>SLINTKIKPFKNQAFKNGEFIEVTEKDTEGRWSVFFFYPADFSFVCPTELGDVADHYEELQKLGVDVYSVSTDTHFTHKAWHSSSETIAKIKYAMIGDPTGALTRNFDNMREDEGLADRATFVVDPQGIIQ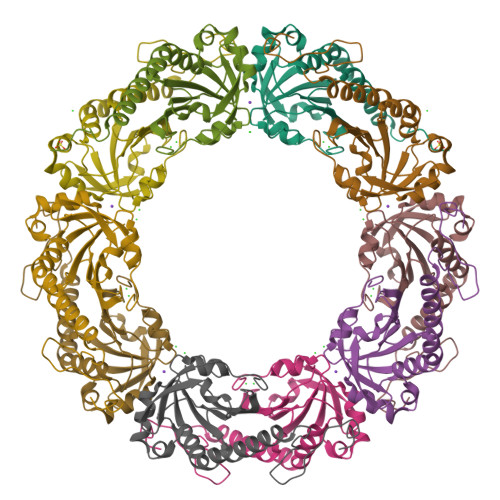AIEVTAEGIGRDASDLLRKIKAAQYVAAHPGEVCPAKWKEGEATLAPSLDLVGKI[5x]>[8x]ARKCSLTGKWTNDLGSNMTIGAVNSRGEFTGTYITAVTATSNEIKESPLHGTQNTINKRTQPTFGFTVNWKFSESTTVF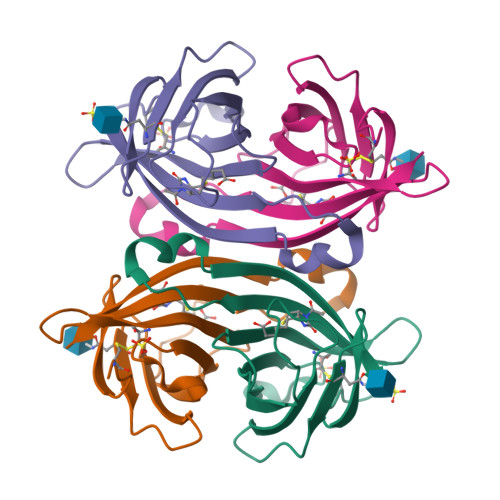TGQCFIDRNGKEVLKTMWLLRSSVNDIGDDWKATRVGINIFTRL> MDLVDRAQAGEAEAFGRLYDQYSDTVYRYIYYRVGGKATAEDLTSETFLRALRRISTFTWQGRDFGAWLVTIARNLVADHFKSMESLSNAALLDAVRRLNPQQQECVTLRFLQGLSVAETARVMGKNEGAIKTLQYRAVRTLARLLPDDAR;> MIANVSAHRRANAFAQALEDRESEGAAAEQTETTAEPAEQGKLLALASGLG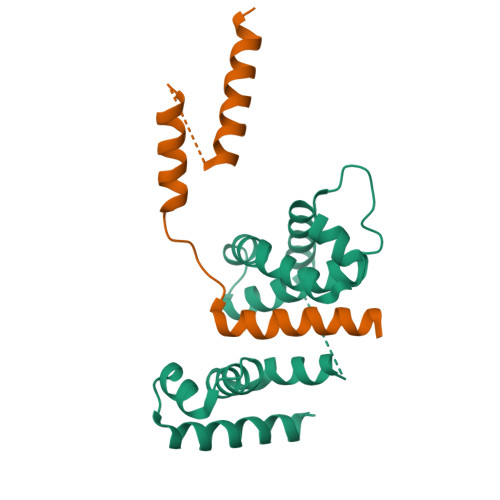DLPKPQLDPEVKVVQRAQLVAAMEAMLMEGSAAAAPTVPE>SNAEKSRSSWIKQLNASLDEIDPEVADIIELEKARQWKGFELIPSENFTSLSVMQAVGSVMTNKYSEGYPGARYYGGNEYIDMAETLCQKRALEAFQLDPSKWGVNVQSLSGSPANFQVYTALLKPHERIMALDLPHGGHLSHGYQTDTKKISAVSIFFETMPYRLDENTGYIDYDQLEKSAVLFRPKLIVAGASAYARLYDYARIRKVCNKQKAVMLADMAHISGLVAAGVIPSPFEYADVVTTTTHKSLRGPRGAMIFFRKGLKEINKQGKEVMYDYEDRINQAVFPGLQGGPHNHTITGLAVALKQARTPEYKAYQD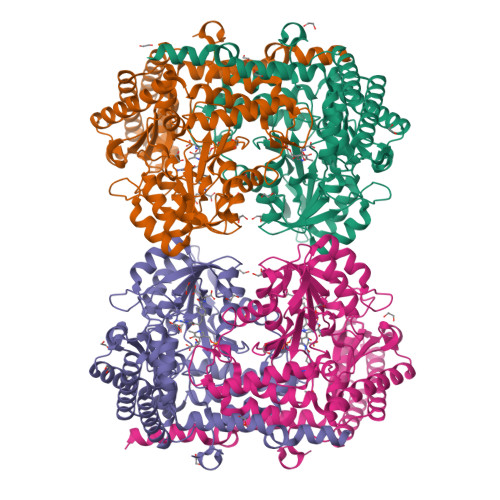QVLRNCSKFAETLLAKGYDLVSGGTDNHLVLVNLKNKGIDGSRVEKVLELVHIAANKNTVPGDVSAMVPGGIRMGTPALTSRGFIEEDFAKVAEYFDLAVKIALKIKAESQGTKLKDFVATMQSNEKLQSEMSKLREMVEEYAKQFPTIGFEKETMRYKE[4x]> MRGSHHHHHHGMASMSVSTASTEMSVRKIAAHMKSNPNAKVIFMVGAGISTSCGIPDFRSPGTGLYHNLARL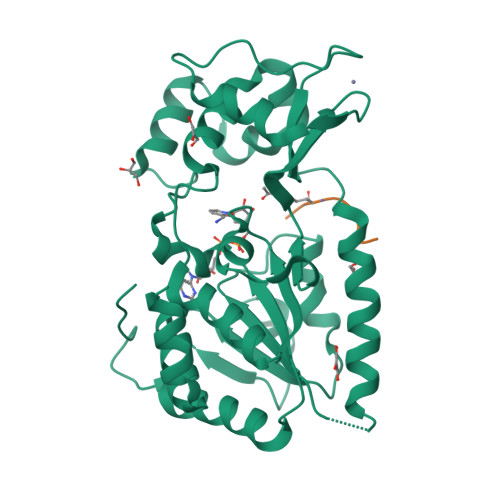KLPYPEAVFDVDFFQSDPLPFYTLAKELYPGNFRPSKFHYLLKLFQDKDVLKRVYTQNFDTLERQAGVKDDLIIEAHGSFAHCHCIGCGKVYPPQVFKSKLAEHPIKDFVKCDVCGELVKPAIVFFGEDLPDSFSETWLNDSEWLREKITTSGKHPQQPLVIVVGTSLAVYPFASLPEEIPRKVKRVLCNLETVGDFKANKRPTDLIVHQYSDEFAEQLVEELGWQEDFEKILTAQ;> KGGAKRHRKILTAQ> QTA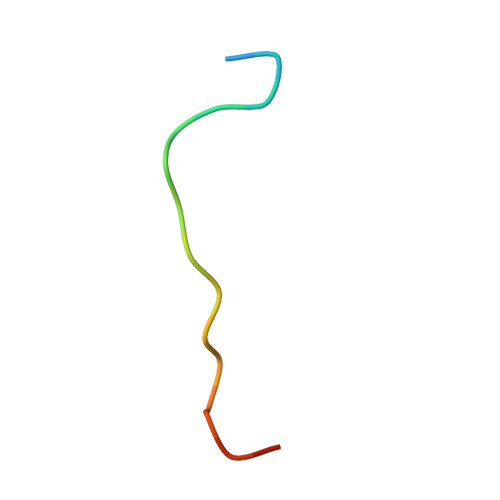RKSTGGKAPRKQLASK8-[4-[2-(4-propanoylpiperazin-1-yl)ethyl]pyrazol-1-yl]-3~{H}-pyrido[3,4-d]pyrimidin-4-one | C19 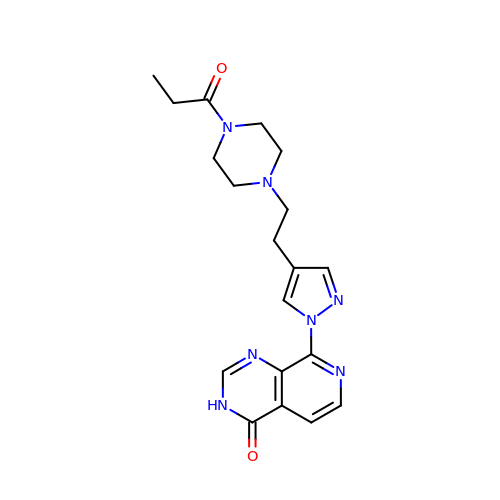H23 N7 O2 | NWZZGCCTCMQFDY-UHFFFAOYSA-N> MSNKEKQMNLLSDKNVAIIGGGPVGLTMAKLLQQNGIDVSVYERDNDREARIFGGTLDLHKGSGQEAMKKAGLLQTYYDLALPMGVNIADEKGNILSTKNVKPENRFDNPEINRNDLRAILLNSLENDTVIWDRKLVMLEPGKKKWTLTFENKPSETADLVIIANGGMSKVRKFVTDTEVEETGTFNIQADIHHPEVNCPGFFQLCNGNRLMAAHQGNLLFANPNNNGALHFGISFKTPDEWKNQTQVDFQNRNSVVDFLLKEFSDWDERYKELIRVTSSFVGLATRIFPLGKSWKSKRPLPITMIGDAAHLMPPFAGQGVNSGLMDALILSDNLTNGKFNSIEEAIENYEQQMFIYGKEAQEESTQNEIEMFKPDFTFQQLLNV

Recently, several plasmid-encoded variants of the tetracycline-degrading enzyme Tet(X), such as Tet(X4) which confers high-level tigecycline resistance, were found to be produced by MDR bacteria isolated from animals and humans. These novel enzymes degrade tetracyclines more effectively than Tet(X). In this study, we characterized the mechanism underlying the degradation of tigecycline by Tet(X4), resolved the crystal structure of the Tet(X4) and tigecycline-Tet(X4) complex, and revealed the substrate basis of Tet(X4)-mediated catalysis.

The monomer includes 369 amino acids of Tet(X4) (Asn247, Gln248, and Thr249 were not modeled), namely, Asn12 to Gln383. In the Tet(X4) and Tet(X4)-tigecycline structures, FAD is bound non-covalently to an IN-conformation such as those of Tet(X) and Tet(X7). The FAD-binding residues (Val27, Glu46, Arg47, Gly57, Gly58, Arg117, Leu139, Asp311, Pro318, and Val324) are conserved in Tet(X2) and Tet(X4). Superimposition of the structure of Tet(X4) and structure of Tet(X2) revealed the difference between the substrate-binding domain of the two enzymes. First, α10 and α11 in the Tet(X4) structure were shorter when compared to Tet(X2), indicating that the loop between α10 and α11 was extended to allow accommodation of a more flexible conformation. The loop has been considered the substrate-binding site; hence, an extended loop might enhance the chance by which tigecycline attaches to FAD for oxidization. In addition, a number of alpha helixes in Tet(X4), namely α6, α7, α8, and α9, have collapsed to generate more loops for substrate binding. α4 formed an alpha helix structure in the Tet(X2) structure, but it was deconstructed as a loop in Tet(X4) structure. As the main components of the substrate-binding domain, β12 and β16 in Tet(X4) have also become smaller in size, forming a larger number of loops when compared to Tet(X2). These structural alterations allowed the secondary structure of Tet(X4) to adopt more loops and turns, rendering the structure of the substrate-binding domain more flexible and more readily to accommodate the tetracycline molecule, resulting in increased catalytic efficiency of enzyme on tigecycline.>DSANLTNRGLVERARRVTAAENYDIGTRFSAMIQSGEGAWLTDVEGNRYVDLTASSGTIILGHRNQAVTEAITRQIRDFGTAFASTLSVPRVELAERLCERYECAEKVVFHKTGSEGTAMAARLARAATGRELILSCGYHGWHEWQLAGETFGYQQTTGVVGFGYNEKALAKMLEAFGNEVAGVLISPELLYFDVEFYQRMYALCARYDVPFMMDEVYTGFRAGPKGVHGLGVPADVVVVSKGLANGHSLAAVMGRRDIIDAYDVSGIQGTYTREVPPMAAAMAVLDVLDTPGVYEHAEAMGRRLADGMREILTGEGIPNWVGGPALMFDTVLPNDDLGWEIYKTAHD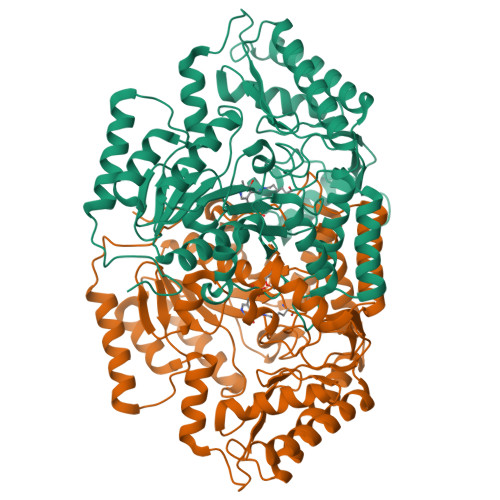FGVYFEDSGTQLVTTAFDEAAVDHALTAFRKATRQVIADRPDIAPTSGGELTEERKLDFAEEAFGGLLRDDERTNALIDETIEKVVNRDRSIKPVLIPAQN[2x]> TSSANEDMPVERILEAELAVEP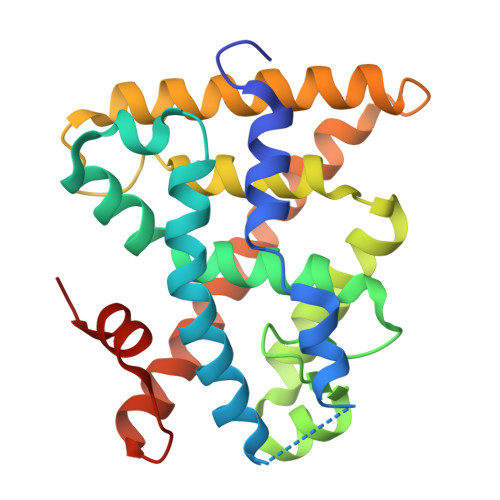KTETYVEANMGLNPSSPNDPVTNICQAADKQLFTLVEWAKRIPHFSELPLDDQVILLRAGWNELLIASFSHRSIAVKDGILLATGLHVHRNSAHSAGVGAIFDRVLTELVSKMRDMQMDKTELGCLRAIVLFNPDSKGLSNPAEVEALREKVYASLEAYCKHKYPEQPGRFAKLLLRLPALRSIGLKCLEHLFFFKLIGDTPIDTFLMEMLEAPHQMT> MIKVEIKPSQAQFTTR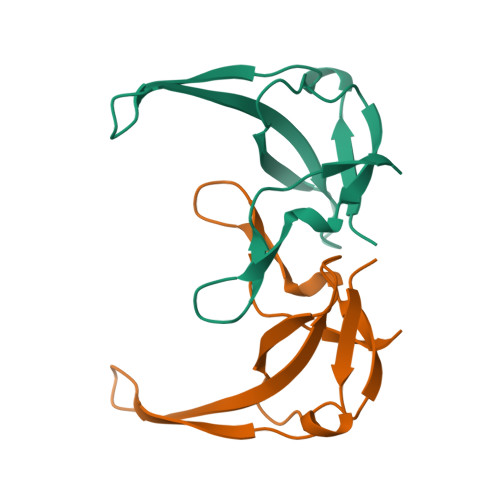SGVSRQGKPYSLNEQLCYVDLGNEYPVLVKITLDEGQPAYAPGLYTVHLSSFKVGQFGSLMIDRLCLVPA>[5x]MTDFDSLSGTSTTWVNELGSVMTIDVDRKGGVTGYYVNNAPGTGCRGLPYDLSGH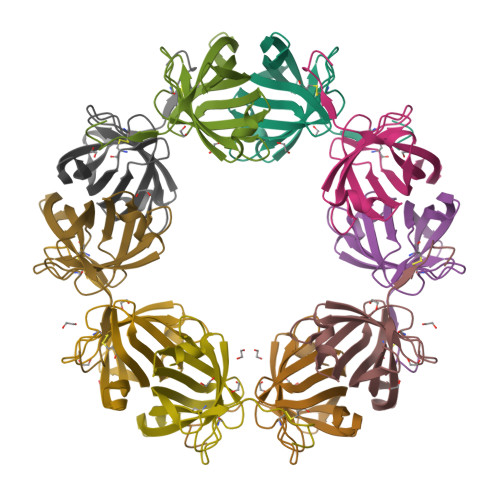AHGSTIAFSVVWSNGIADCRSATSWAGYARKTFGGGVQIVTQWSLAFVGKAGGKIETGQNVFTYQAATVSESLLTE2-fluoro-6-{[2-({2-methoxy-4-[4-(1-methylethyl)piperazin-1-yl]phenyl}amino)-7H-pyrrolo[2,3-d]pyrimidin-4-yl]amino}benzamide | C27 H31 F N8 O2 | 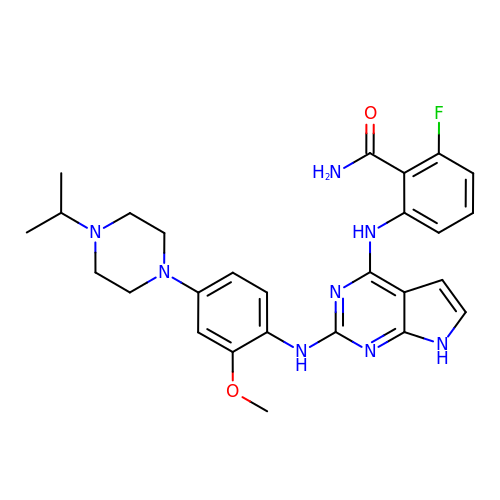HXZDICYKFAOZLE-UHFFFAOYSA-N>QDNSRYTHFLTQHYDAKPQGRDDRYCESIMRRRGLTSPCKDINTFIHG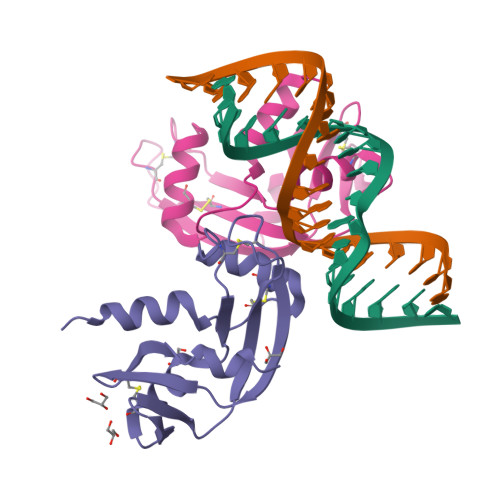NKRSIKAICENKNGNPHRENLRISKSSFQVTTCKLHGGSPWPPCQYRATAGFRNVVVACENGLPVALDQSIFRRP[2x]>GAMADIAHEIRTPITNLITQTEIALSQSRSQKELEDVLYSNLEELTRMAKMVSDMLFLAQADNNQLIPEKKMLNLADEVGKVFDFFEALAEDRGVELRFVGDKCQVAGDPLMLRRALSNLLSNALRYTPPSEAIVVRCQTVNHQVQVSVENPGTPIAPEHLPRLFDRFYRVAPSRQ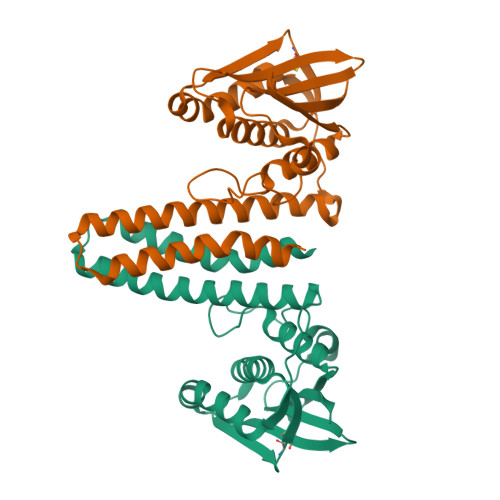RKGEGSGIGLAIVKSIVVAHKGTVAVTSDARGTRFVITLPA[6x]> MPTITPNKLTLKIGRAEGRPGDTVEIPVNLYGVPQKGIASGDFVVSYDPNVLEIIEIEPGELIVDPNPTKSFDTAVYPDRKMIVFLFAEDSGTGAYAITEDGVFATIVAKVKEGAPEGFSAIEISEFGAF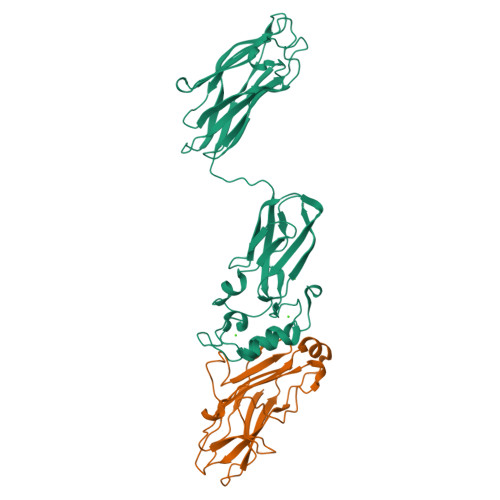ADNDLVEVETDLINGGVLVTNKPVIEGYKVSGYILPDFSFDATVAPLVKAGFKVEIVGTELYAVTDANGYFEITGVPANASGYTLKISRATYLDRVIANVVVTGDTSVSTSQAPIMMWVGDIVKDNSINLLDVAEVIRCFNATKGSANYVEELDINRNGAINMQDIMIVHKHFGATSSDYDAQLEHHHHHH;> MRGSHHHHHHTDLRADKASSIELKFDRNKGEVGDILIGTVRINNIKNFAGFQVNIVYDPKVLMAVDPETGKEFTSSTFPPGRTVLKNNAYGPIQIADNDPEKGILNFALAYSYIAGYKETGVAEESGIIAKIGFKILQKKSTAVKFQDTLSMPGAISGTQLFDWDGEVITGYEVIQPDVLSLGDEPY2-hydroxy-4-(2-hydroxyethyl)phenyl beta-D-fructofuranoside 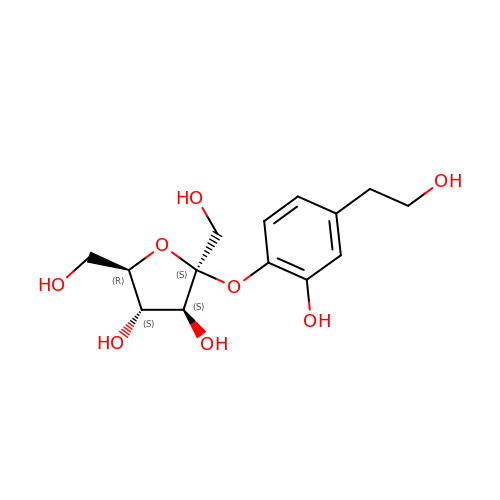| C14 H20 O8 | CNXXGYXVIZNKJW-YIYPIFLZSA-N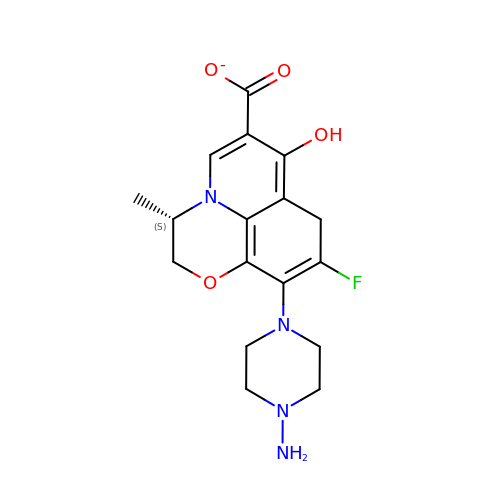(3S)-10-(4-AMINOPIPERAZIN-1-YL)-9-FLUORO-7-HYDROXY-3-METHYL-2,3-DIHYDRO-8H-[1,4]OXAZINO[2,3,4-IJ]QUINOLINE-6-CARBOXYLATE | C17 H19 F N4 O4 | XSSSNYCVNIDBIB-VIFPVBQESA-M>APIKVGINGFGRIGRMVFQAICDQGLIGTEIDVVAVVDMSTNAEYFAYQMKHDTVH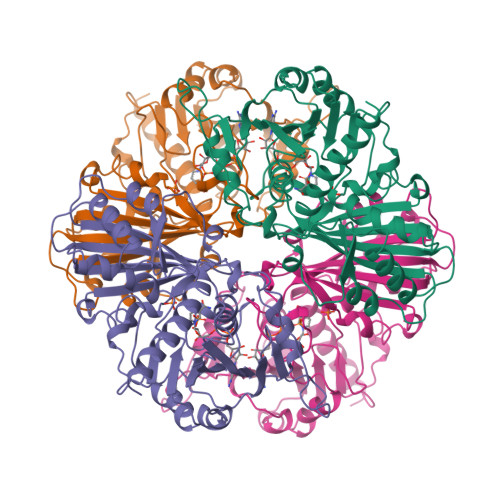GRPKYTVEAVKSSPSVETADVLVVNGHRIKCVKAQRNPADLPWGKLGVDYVIESTGLFTDKLKAEGHIKGGAKKVVISAPASGGAKTIVMGVNQHEYSPASHHVVSNASCTTNCLAPIVHVLTKENFGIETGLMTTIHSYTATQKTVDGVSLKDWRGGRAAAVNIIPSTTGAAKAVGMVIPSTKGKLTGMSFRVPTPDVSVVDLTFRATRDTSIQEIDKAIKKAAQTYMKGILGFTDEELVSADFINDNRSSVYDSKATLQNNLPGEKRFFKVVSWYDNEWAYSHRVVDLVRYMAAKDAASSKM[4x]>[2x]SMIKENVYFDGNVKSLGFSQQDG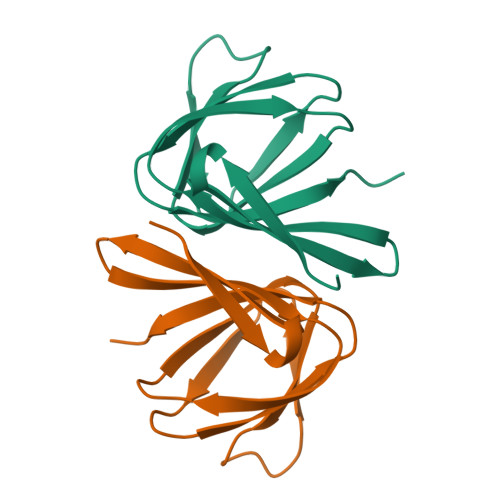ESTVGVMAPGQYTFGTGAPERMTVVKGALTIKRVTDADWVTFTAGEAFEVAGNSSFDLQVEVATAYLCEFLPA>MLAVLEIGIIENVQRADLNVLEEALSYKVLMEKFERTQENIAQTIGKSRSHVANTMRLLALPDEVQSYLVSGELTAGHARAIAAAADPVALAKQIIEGGLSVRETEALARKAPNLSAGKSKGGRPPRVKDKLAAALEHHHHHH[2x]

Using a pair of evolutionarily related DNA-binding proteins, each with a different DNA preference (ParB [Partitioning Protein B] and Noc [Nucleoid Occlusion Factor], which both play roles in bacterial chromosome maintenance), we show that specificity is encoded by a set of four residues at the protein-DNA interface. Like ParB, Noc has a three-domain architecture: an N-terminal domain for protein-protein interactions and for targeting Noc to the cell membrane, a central DNA-binding domain (DBD), and a C-terminal dimerization domain (Wu and Errington, 2004; Wu et al., 2009). The NBS site differs from the parS site by only 2 bases (positions 1 and 6), but Noc and ParB recognize and bind them with exquisite specificity. We show that specificity to parS or NBS is encoded by a small set of four residues at the protein-DNA interface and that mutations in these residues are enough to reprogram DNA-binding specificity.

As the first step in identifying specificity residues, we solved a 2.4-Å resolution co-crystal structure of the DBD of Caulobacter crescentus ParB bound to a 20-bp parS DNA duplex. In the crystallographic asymmetric unit, two very similar ParB DBD monomers (root-mean-square deviation [RMSD] = 0.1 Å) bind in a 2-fold symmetric fashion to a full-size parS DNA duplex. This structure reveals several regions of each DBD that contact parS. First, the recognition helix α4 of the helix-turn-helix motif inserts into the major grooves of the palindromic parS site. Second, helices α6 and α8 contribute residues to the protein-DNA interface. Last, several lysine and arginine residues in the loop spanning residues 236–254 contact the minor groove side of parS in an adjacent complex in the crystal. We found that most of the crucial residues for binding to parS are within the 162–234 region, suggesting their importance in recognizing DNA specifically. First, R173 in ParB hydrogen bonds with parS guanine 1, but the shorter side chain of a corresponding Q158 in Noc is unable to bond with guanine 1. G201 from ParB has no side chain and hence cannot contact thymine −6 specifically.>[2x]MAHHHHHHMSTQAAMTTAERWQKIQAQAPDVIFDLAKRAAAAKGPKANLVIGAYRDEQGRPYPLRVVRKAEQLLLDMNLDYEYL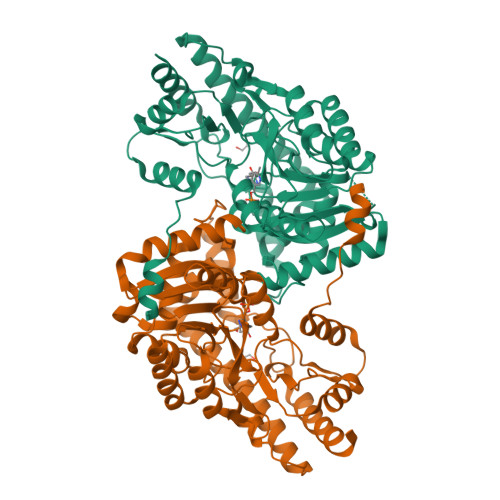PISGYQPFIDEAVKIIYGNTVELENLVAVQTLSGTGAVSLGAKLLTRVFDAETTPIYLSDPTWPNHYGVVKAAGWKNICTYAYYDPKTVSLNFEGMKKDILAAPDGSVFILHQCAHNPTGVDPSQEQWNEIASLMLAKHHQVFFDSAYQGYASGSLDTDAYAARLFARRGIEVLLAQSFSKNMGLYSERAGTLSLLLKDKTKRADVKSVMDSLIREEYTCPPAHGARLAHLILSNNELRKEWEAELSAMAERIRTMRRTVYDELLRLQTPGSWEHVINQIGMFSFLGLSKAQCEYCQNHNIFITVSGRANMAGLTHETALMLAQTINDAVRNVNRE> A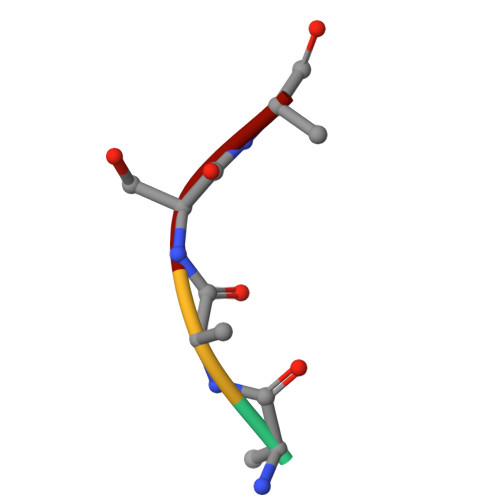LSR>[10x]LDRADILYNIRQTSRPDVIPTQRDRP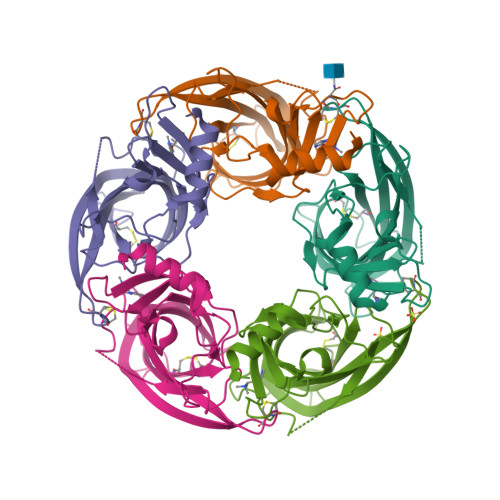VAVSVSLKFINILEVNEITNEVDVVFWQQTTWSDRTLAWNSSHSPDQVSVPISSLWVPDLAAYNAISKPEVLTPQLARVVSDGEVLYMPSIRQRFSCDVSGVDTESGATCRIKIGSWTHHSREISVDPTTENSDDSEYFSQYSRFEILDVTQKKNSVTYSCCPEAYEDVEVSLNFRKKGRSEIL Formate de­hydrogenases (FDHs) catalyze the two-electron oxidation of formate to carbon dioxide and play an important role in several kingdoms of organisms. The second class of enzymes is metal-dependent (Mo- or W-containing) FDHs from prokaryotic organisms, which belong to the superfamily of molybdenum enzymes and are members of the di­methyl­sulfoxide (DMSO) reductase family. The metal-containing formate de­hydrogenase 1 from M. extorquens AM1 (MeFDH1) comprises two subunits and is located in the cytoplasmic fraction.

Recently, we successfully determined the structure of MeFDH1, a W–Cys-type enzyme, by means of cryo-EM and X-ray crystallography. MeFDH1 consists of two subunits denoted α and β [Fig. 1(a)]. The α subunit contains the W–Cys active site with the proximal [4Fe–4S] cluster, along with an additional two [4Fe–4S] clusters and one [2Fe–2S] cluster. The β subunit harbors the binding site for NAD+ and possesses one FMN cofactor, one [4Fe–4S] cluster and one [2Fe–2S] cluster. The [4Fe–4S] cluster in the β subunit is connected to the [4Fe–4S] and [2Fe–2S] clusters in the α subunit with distances of 14.9 and 10.9 Å, respectively. The β subunit is responsible for catalyzing the NAD+/NADH redox couple in MeFDH1 and is therefore called the diaphorase unit. The structure of W–Cys-type MeFDH1 is also very similar to that of Mo–Cys-type RcFdsGBACD [RcFDH homologously expressed in R. capsulatus with operon fdsGBACD], although the orientation of the β subunit with respect to the α subunit is slightly different. The cryo-EM structure of Mo–Cys-type RcFdsGBACD revealed that the Mo ion was coordinated by six ligands of the bis-MGD cofactor, the cysteine sulfur and a sulfido ligand with similar geometry to the other FDHs. The recent structural analysis of W–Cys-type MeFDH1 in the oxidized state showed, however, that the six ligands coordinated to the W ion were those from the bis-MGD, a cysteine sulfur and a tentative oxygen species based on the coordination bond lengths. A highly conserved lysine residue (K44 in EcFDH-F and K331 in MeFDH1) is located between the pterin cofactor and the proximal [4Fe–4S] cluster.

> MSNGPEPHGNKIEQPEIRADERQDAGGPANGAPSTSGGAYSQGAKSGGQAAPDPSGSYGIKDAPVAPATIAFEFDGQQVEAQPGETIWAVAKRLGTHIPHLCHKPDPGYRPDGNCRACMVEIEGERVLAASCKRTPAIGMKVKSATERATKARAMVLELLVADQPERATSHDPSSHFWVQADVLDVTESRFPAAERWTSDVSHPAMSVNLDACIQCNLCVRACREVQVNDVIGMAYRAAGSKVVFDFDDPMGGSTCVACGECVQACPTGALMPAAYLDANQTRTVYPDREVKSLCPYCGVGCQVSYKVKDERIVYAEGVNGPANQNRLCVKGRFGFDYVHHPHRLTVPLIRLENVPKDANDQVDPANPWTHFREATWEEALDRAAGGLKAIRDTNGRKALAGFGSAKGSNEEAYLFQKLVRLGFGTNNVDHCTRLCHASSVAALMEGLNSGAVTAPFSAALDAEVIVVIGANPTVNHPVAATFLKNAVKQRGAKLIIMDPRRQTLSRHAYRHLAFRPGSDVAMLNAMLNVIVTEGLYDEQYIAGYTENFEALREKIVDFTPEKMASVCGIDAETLREVARLYARAKSSLIFWGMGVSQHVHGTDNSRCLIALALITGQIGRPGTGLHPLRGQNNVQGASDAGLIPMVYPDYQSVEKDAVRELFEEFWGQSLDPQKGLTVVEIMRAIHAGEIRGMFVEGENPAMSDPDLNHARHALAMLDHLVVQDLFLTETAFHADVVLPASAFAEKAGTFTNTDRRVQIAQPVVAPPGDARQDWWIIQELARRLDLDWNYGGPADIFAEMAQVMPSLNNITWERLEREGAVTYPVDAPDQPGNEIIFYAGFPTESGRAKIVPAAIVPPDEVPDDEFPMVLSTGRVLEHWHTGSMTRRAGVLDALEPEAVAFMAPKELYRLGLRPGGSMRLETRRGAVVLKVRSDRDVPIGMIFMPFCYAEAAANLLTNPALDPLGKIPEFKFCAARVVPAEAAPMAAE;> MSEASGTVRSFAHPGRGRNVARAVPKGRQVDPHAKVEIEELLGTRPRQRDLLIEHLHLIQDTYGQISADHLAALADEMSLAFAEVFETATFYAHFDVVKEGEADIPRLTIRVCDSITCAMFGADELLETLQRELASDAVRVVRAPCVGLCDHAPAVEVGHNFLHRADLASVRAAVEAEDTHAHIPTYVDYDAYRAGGGYATLERLRSGELPVDDVLKVLDDGGLRGLGGAGFPTGRKWRSVRGEPGPRLMAVNGDEGEPGTFKDQLYLNTDPHRFLEGMLIGAHVVEAADVYIYLRDEYPISREILAREIAKLPEGGTRIHLRRGAGAYICGEESSLIESLEGKRGLPRHKPPFPFQVGLFNRPTLINNIETLFWVRDLIERGAEWWKSHGRNGRVGLRSYSVSGRVKEPGVKLAPAGLTIQELIDEYCGGISDGHSFAAYLPGGASGGILPASMNDIPLDFGTLEKYGCFIGSAAVVILSDQDDVRGAALNLMKFFEDESCGQCTPCRSGTQKARMLMENGVWDTDLLGELAQCMRDASICGLGQAASNPVSTVIKYFPDLFPEPRAVAAE In this study, we look at how a mitochondrial homolog of the molecular chaperone Hsp90 (TRAP1)2 may be regulated by calcium binding via a novel mechanism. All Hsp90s are homodimers with each protomer composed of 3 globular domains: an ATP-binding N-terminal domain (NTD), a middle domain, and C-terminal dimerizing domain (CTD). TRAP1 structural studies have revealed the presence of a remarkably asymmetric closed state in the presence of nonhydrolyzable ATP analogs that leads to a two-step sequential ATP hydrolysis mechanism, with the first ATP leading to a flip in asymmetry, and the second leading to re-opening. We found that unlike most other Hsp90 homologs, the TRAP1 ATPase can efficiently utilize calcium alone to support hydrolysis, and that the relative preference for magnesium or calcium depends upon the concentration of free ATP.

To determine where calcium binds in the closed state and any consequences on the structure, we replaced the magnesium in our standard zTRAP1 crystallization conditions with calcium. Despite the similarity in overall structure, no density coordinating the β- and γ-phosphates, where magnesium would be, was observed. To unambiguously determine where calcium binds, we exploited the anomalous X-ray scattering signal from calcium and collected two datasets: one at 7450 eV (1.664 Å) and 11111 eV (1.116 Å). Using phases from the solved structure without the contribution of calcium atoms, the resulting anomalous difference density map reveals one strong peak within the nucleotide pocket of each protomer, located just above the α-phosphate (inset). The density is tightly coordinated by six oxygen atoms in an octahedral arrangement near the “lid” of the NTD (4 backbone carbonyl oxygens, a tyrosine hydroxyl, and the α-phosphate). Rather than being a magnesium mimic positioned to stabilize negative charge build-up on the β- and γ-phosphates at the catalytic transition state, direct visualization of the calcium-binding site by crystallography shows that calcium occupies a site near the α-phosphate. In the closed state, the calcium is octahedrally coordinated by backbone carbonyl oxygens from the ATP lid, Tyr-221 hydroxyl, and the ATP α-phosphate oxygen. Unlike the magnesium site, this site is configured quite differently in the apo state versus the closed state, thus providing a unique coupling between open-closed conformation and calcium binding. Structural data supports that the calcium-binding cavity near the α-phosphate presented here is conserved in the GHKL (Gyrase, Hsp90, histidine Kinase and MutL) ATPase superfamily. The remarkable change in cooperativity observed with calcium indicates that TRAP1 can adopt a switch-like response to calcium at high ATP levels, providing a strong connection between calcium concentration in the mitochondrial matrix and TRAP1 ATPase-driven cycling.

>TLHNIITDTENVQGSFSKHEFQAETKKLLDIVARSLYSEKEVFIRELISNGSDALEKLRHRMITAGGDTAPMEIHLQTDSVKGTFTIQDTGVGMNKEDLVSNLGTIARSGSKAFLDALQNQAEASSSIIGQFGVGFYSAFMVADKVEVYSQSAEADAPGYKWSSDGSGVFEVAEASGVRQGTKIVLHLKDDCKEFSSEDRVKEVVTKYSNFVSFPIFLNGRRLNTLQALWMMEPKDISEWQHEEFYRYVAQAYDKPRYTLHYRADAPLNIRSIFYVPEMKPSMFDVSREMGSSVALYSRKILIQTKATDILPKWLRFLRGVVDSEDIPLNLSRELLQESALIRKLRDVLQQRVIRFLLDQSKKDPEKYARFFEDYGLFMREGIVTTGEQSVKEDIAKLLRFESSALPAGQQTSLMEYSSRMKAGTRNIYYLCAPNRHLAEHSPYFEAMKQKDMEVLFCFEQFDELTLLHLREFDRKKLISAETDIVVDHYKEEKFQDSKPASERLSSEQAEDLLAWMRNALVQRVTNIKVTPRLDTHPAMITVLEMGAARHFLRTQQLARSSEERAQILQPTLEINTGHDLIKKLHALKDSNPELAQLLLEQIYDNAMIAAGLNEDPRPMISRLNQLLTRALEKH[2x]> QLQQQEDDRILGLPGQPNGVAFGMYGGYVTIDDNNGRALYYWFQEADTADPAAAPLVLWLNGGPGCSSIGLGAMQELGAFRVHTNGESLLLNEYAWNKAANILFAESPAGVGFSYSNTSSDLSMGDDKMAQDTYTFLVKWFERFPHYNYREFYIAGESGHFIPQLSQVVYRNRNNSPFINFQGL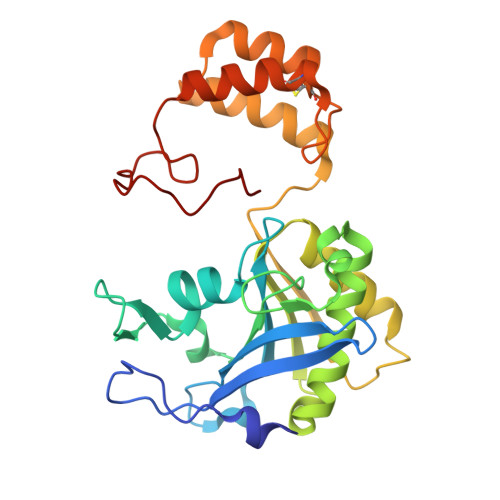LVSSGLTNDHEDMIGMFESWWHHGLISDETRDSGLKVCPGTSFMHPTPECTEVWNKALAEQGNINPYTIYTPTCDREPSPYQRRFW> SNAMDLVQKQKSL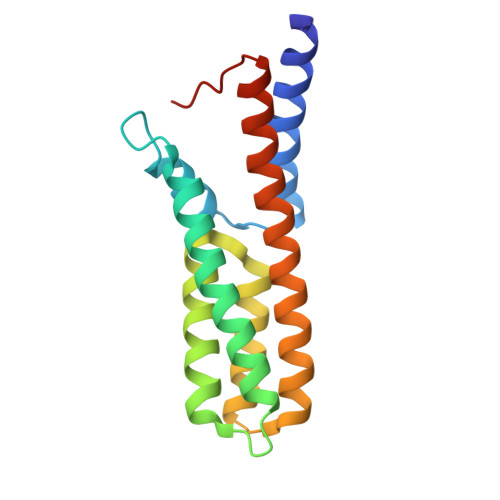QDYTKSLFLEGILDSQFLQLQQLQDESNPDFVSQVVTLFFQDSDRILNDLSLSLDQQVVDFKKVDPHVHQLKGSSSSIGAQRVKNACVVFRSFCEQQNVEACHRCLQQVKQEYYLVKNRLETLFKLEQQIVASGGMIPAVELGF>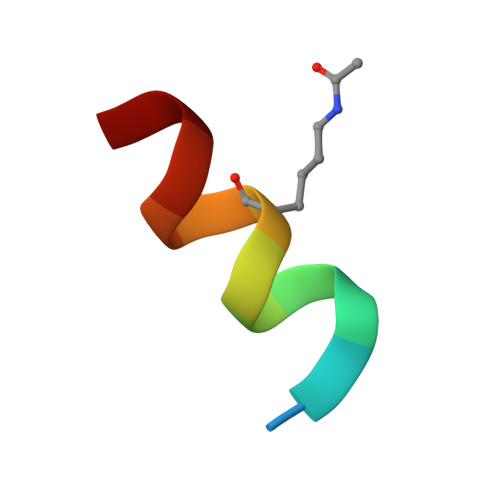 XWSWLCKKYNLIH(5S)-7-(pyrazin-2-yl)-2-oxa-7-azaspiro[4.4]nonane | C11 H15 N3 O | 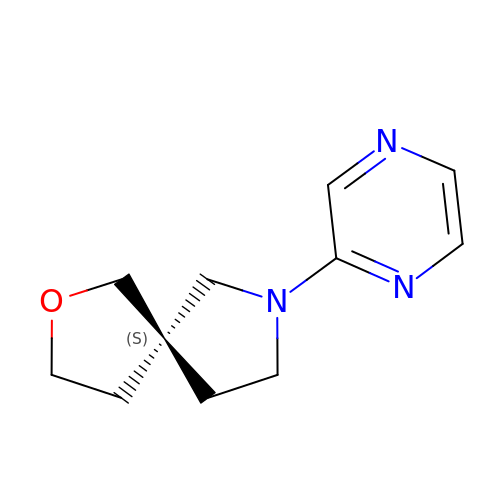ITTBXBSSJHVWJS-NSHDSACASA-N> NKTHQVEHESEQSDFQDIRFGLNSVKLPKAQPAAATRITVENGTDKLVNYKSSPQQLFLAKNALKDKLQGEFDKFLSDAKAFPALTADLQEWVDQQLFNPNQSFFDLSAPRSNFTLSSDKKASLDFIFRFTNFTESVQLLKLPEGVSVVVDSKQSFDYYVNASAQKLLVLPLSLPDYTLGLNYMFDHITLNGKVVNKFSFNPFKTNLNLAFSNVYNGVDVFEAQKNLVGKGKYLNTHVKAEDVKKDVNANIKNQFDIAKIIAELMGKALKEFGNQQEGQPLSFLKVMDKVKEDFEKLFNLVRPGLGKFVKDLIQSSSQAENKITVYKLIFDNKKTILNLLKELSIPELNSSLGLVDVLFDGITDSDGLYERLQSFKDLIVPAVKTNEKTAALSPLIEELLTQKDTYVFDLIQKHKGILTNLLKNFLADFQKSTPFMADQVAIFTELFDNEGAFDLFGEADFVDKIAELFLTKRTVKNGEKIETKDSLLVTSLKSLLGEKVAALGDLLDSYIFKNELLNRSVEVAKAEAKDTKGATDYKKEQAKALKKLFKHIGENTLSKTNLDKITLKEVKNTENVELEETETTLKVKKLDVEYKVELGNFEIKNGLIKAMLEFLPDTKDLETTLDKLLFKGESYKAMKDKYIKEGFPGYGWAKGVVPGAFESIENTFKSAIDKTKSIRDLFGDMLFGNDLSSVKETDSFITLGGSFDIKYGGENLNVLPAYYSLINSEIGYQIIGVDTTIDATKVKVELKNKEYKGKSPAINGQVKLSQSFFNVWTNMFDSITKQIFQKKYEFKDNIQVFARNEDNTSRLELDISDPEQRVIPFAFVDGFGIQLKAVDKNITKEAGNTEPKSPVIQLYEALNKEKDQKQQSKQSPKQLDTKTQLGYLLKLGDNWSKDDYKSLIDDTIINNNYLEASFNSKITVDRLGIPIDLWLFKIWPKFNLEIPMQGSLQLYSSSVIFPYGIYDTSVQDAAKIVKRLNFTDMGFKLNDPKPNFWFVGFKHHHHH

Here, we report a comprehensive structural and functional analysis of the previously uncharacterized protein P116 (MPN_213). Single-particle cryo-electron microscopy of P116 reveals a homodimer presenting a previously unseen fold, forming a huge hydrophobic cavity, which is fully accessible to solvent. Lipidomics analysis shows that P116 specifically extracts lipids such as phosphatidylcholine, sphingomyelin and cholesterol. Each monomer consists of two distinct domains: the core domain (residues 246–867) and the amino-terminal domain (residues 60–245), situated distal to the dimer axis.

To obtain empty P116 that is free of any bound ligands, we treated the P116 samples with the detergent Triton X-100. Mass spectrometry confirmed a massive reduction of lipids in the sample. The structure of the empty P116 sample was solved by cryoEM at 4-Å resolution. Its overall topology is almost identical to that of the original P116 sample; however, the core domain is constricted as a result of fingers 1, 2 and 3 being closer to the palm by 8, 13 and 12 Å, respectively, and finger 4 moving 11 Å sideways to retain the distal core access to the cavity. Consequently, the huge hydrophobic cavity reduces to two pockets that are large enough for lipids to pass through but that appear unoccupied in the cryoEM density. A comparison of the filled and empty P116 structures shows that the original densities that were unaccounted for create massive steric clashes in the constricted configuration, demonstrating that the cavity can no longer accommodate lipids. In the empty P116, the dimerization interface is shifted towards the dorsal side of the molecule by 10 Å, resulting in a contraction that changes the arc diameter of the dimer to ~10 nm and shifts the N-terminal domain towards the dimerization interface. Most prominently, the arc diameter of the empty structure is approximately 10 nm smaller than that of the original and refilled structures. In the empty P116, we observed a substantial reduction of lipids, with no specific lipid class enriched.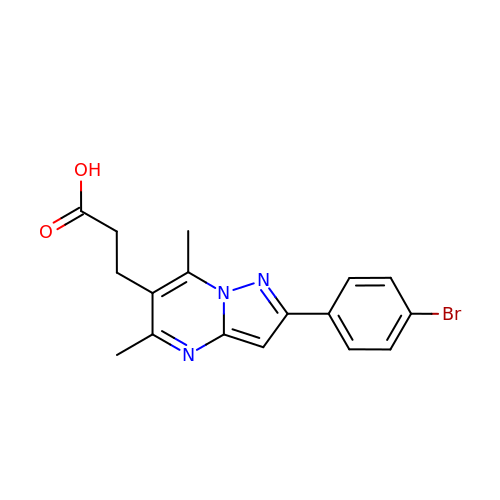3-[2-(4-bromophenyl)-5,7-dimethyl-pyrazolo[1,5-a]pyrimidin-6-yl]propanoic acid | C17 H16 Br N3 O2 | SJELVUFWTXHLTJ-UHFFFAOYSA-N>GSHMSPREQDRFLPIANVSRIMKKALPANAKISKDAKETMQE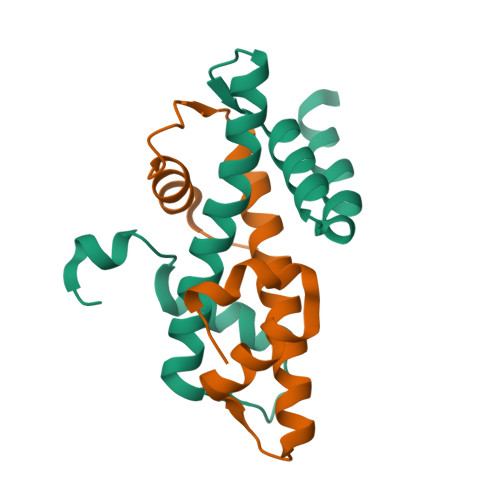CVSEFISFVTGEASDKCQKEKRKTINGDDLLWAMTTLGFEDYVEPLKVYLQRFRE[2x];>[2x]MTQFKEIEKTTDFKNHSLPLARIKKIMKADEDVRMISAEAPVVFARACEMFILELTLRSWNHTEENKRRTLQKNDIAAAVTRTDIFDFLVDIVPR7-({[3-(4-methoxypyridin-3-yl)propyl]amino}methyl)quinolin-2-amine 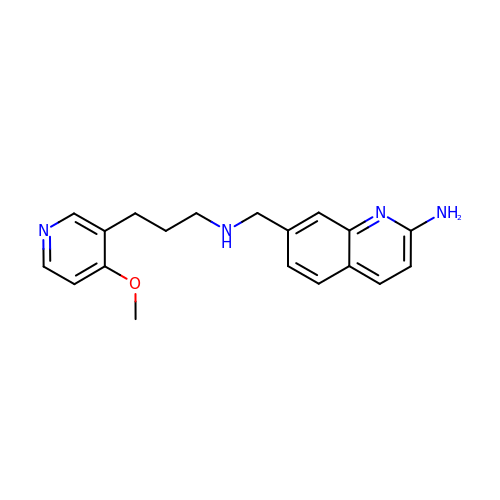| C19 H22 N4 O | IQPCOMIHSUSLGC-UHFFFAOYSA-N>[4x]MHIERLAVDESVGRAMPPQRFIEALSDLGVPVEFAGEDEQFGPGDAVASFGHRDAFLDADWVHCIRAGYDEFPVGVYEEAGTYLTNSTGIHGTTVGETVAGYMLTFARRLHAYRDAQHDHAWDLPRYEEPFTLAGERVCVVGLGTLGRGVVDRAAALGMEVVGVRRSGDPVDNVSTVYTPDRLHEAIADARFVVLATPLTDETEGMVAAPEFETMREDASLVNVARGPVVVESDLVAALDSGDIAGAALDVFSEEPLPEDSPLWDFEDVLITPHVSAATSKYHEDVAALIRENIEKIATGDELTNRVV

Here we describe the molecular basis of the reaction mechanism and dual NADH/NADPH-specificity of D2HDH, a 2-hydroxyacid dehydrogenase from the extreme halophile Haloferax mediterranei, an organism whose proteins have to remain active in high intracellular concentrations of KCl. Sequence analysis has identified D2HDH as a member of the DDH clade of the D-isomer specific 2-hydroxyacid dehydrogenase enzyme family (2HADH), which has potential applications in the synthesis of chiral fine chemicals including alcohols, and hydroxy or amino acids from ketones or ketoacids. Structural studies have shown that all members of this family share a common fold based on two domains, which cycle between open and closed conformational states that serve to close the inter-domain cleft, bringing the substrates together during catalysis. The D2HDH dimer has an overall ellipsoidal appearance in which each monomer is folded into two domains (d1; residues 1–92 and 283–308 and d2; residues 93–282).

Interestingly, the structures of the D2HDH complexes determined in this study have shown that, dependent upon the crystallisation conditions used, the 2-ketoacid substrate can be trapped in the crystal structure in two different orientations, representing a catalytic or abortive mode of binding. In both the productive and abortive modes of substrate binding the 2-ketohexanoic acid alkyl side chain occupies a similar position in the active site, but is twisted as a result of a 120° rotation to the C2-C3 torsion angle. In this structure the ketoacid was also bound in the abortive orientation, showing that the difference was independent of the nature of the co-factor.>[2x]GPLGSPRYELGEELRDKIKQEPSFSNMVSAKKFYNKAIKDFTAPKEGAEVVSVKTHIMRPIDFMLMGLREEFNLYSEDGAHLSAPGTIRLLREKNLLPEEQIARIESVYNQAMSKRFELHAEHKKEHDEMPY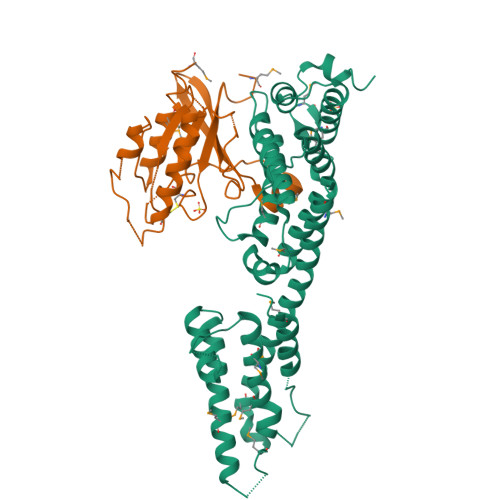SDAKAMLDEVAKIRELGVQRVTRIENLENAKKLWDNANSMLEKGNISGYLKAANELHKFMKEKNLKEDDLRPELSDKTISPKGYAILQSLWGAASDYSRAAATLTESTVEPGLVSAVNKMSAFFMDCKLSPNERATPDPDFKVGKSKILVGIMQFIKDVADPTSKIWMHNTKALMNHKIAAIQKLERSNNVNDETLESVLSSKGENLSEYLSYKYATKDEGREHRYTASTE;>MGSSHHHHHHSSGENLYFQGRPMSSMNPEYDYLFKLLLIGDSGVGKSCLLLRFADDTYTESYISTIGVDFKIRTIELDGKTIKLQIWDTAGQERFRTITSSYYRGAHGIIVVYDVTDQESFNNVKQWLQEIDRYASENVNKLLVGNKCDLTTKKVVDYTTAKEFADSLGIPFLETSAKNATNVEQSFMTMAAEIKKRMG[2x]>[2x]MNPAAEAEFNILLATDSYKVTHYKQYPPNTSKVYSYFECREKKTENSKLRKVKYEETVF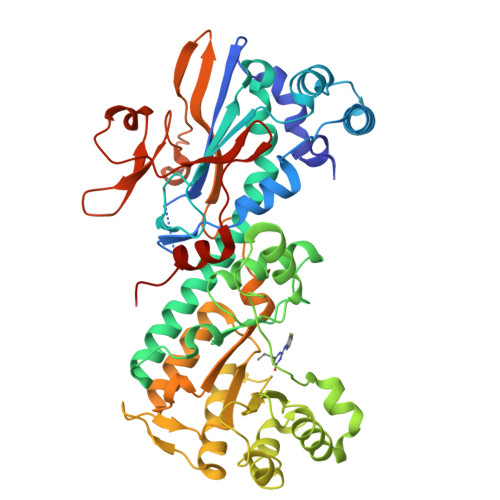YGLQYILNKYLKGKVVTKEKIQEAKDVYKEHFQDDVFNEKGWNYILEKYDGHLPIEIKAVPEGFVIPRGNVLFTVENTDPECYWLTNWIETILVQSWYPITVATNSREQKKILAKYLLETSGNLDGLEYKLHDFGYRGVSSQETAGIGASAHLVNFKGTDTVAGLALIKKYYGTKDPVPGYSVPAAEHSTITAWGKDHEKDAFEHIVTQFSSVPVSVVSDSYDIYNACEKIWGEDLRHLIVSRSTQAPLIIRPDSGNPLDTVLKVLEILGKKFPVTENSKGYKLLPPYLRVIQGDGVDINTLQEIVEGMKQKMWSIENIAFGSGGGLLQKLTRDLLNCSFKCSYVVTNGLGINVFKDPVADPNKRSKKGRLSLHRTPAGNFVTLEEGKGDLEEYGQDLLHTVFKNGKVTKSYSFDEIRKNAQLNIELEAAHH> GPAMCPTHADSLNNLANIKREQGNIEEAVRLYRKALEVFPEFAAAHSNLASVLQQQGKLQEALMHYKEAIRISPTFADAYSNMGNTLKEMQDVQGALQCYTRAIQINPAFADAHSNLASIHKDSGNIPEAIASYRTALKLKPDFPDAYCNLAHCLQIVCDWTDYDERMKKLVSIVADQLEKNRLPSVHPHHSMLYPLSHGFRKAIAERHGNLCLDKINVLHKPPYEHPKDLKLSDGRLRVGYVSSDFGNHPTSHLMQSIPGMHNPDKFEVFCYALSPDDGTNFRVKVMAEANHFIDLSQIPCNGKAADRIHQDGIHILVNMNGY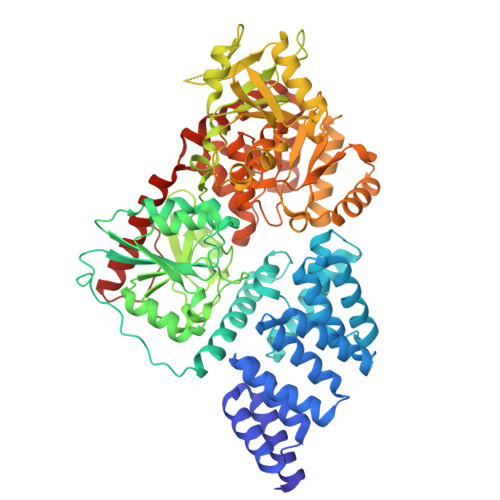TKGARNELFALRPAPIQAMWLGYPGTSGALFMDYIITDQETSPAEVAEQYSEKLAYMPHTFFIGDHANMFPHLKKKAVIDFKSNGHIYDNRIVLNGIDLKAFLDSLPDVKIVKMKCPDGGDNADSSNTALNMPVIPMNTIAEAVIEMINRGQIQITINGFSISNGLATTQINNKAATGEEVPRTIIVTTRSQYGLPEDAIVYCNFNQLYKIDPSTLQMWANILKRVPNSVLWLLRFPAVGEPNIQQYAQNMGLPQNRIIFSPVAPKEEHVRRGQLADVCLDTPLCNGHTTGMDVLWAGTPMVTMPGETLASRVAASQLTCLGCLELIAKNRQEYEDIAVKLGTDLEYLKKVRGKVWKQRISSPLFNTKQYTMELERLYLQMWEHYAAGNKPDHMIKPVE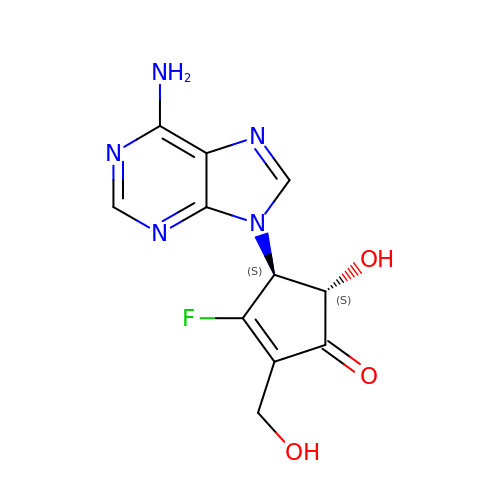(4S,5S)-4-(6-amino-9H-purin-9-yl)-3-fluoro-5-hydroxy-2-(hydroxymethyl)cyclopent-2-en-1-one | C11 H10 F N5 O3 | DMGPQGOOCCLGOU-APPZFPTMSA-N> ATQRKGTDEIYGLGSLPSAGPGRWEYLANPGNWHPERRKLHEKLLDQARSSALTLAESLESDGCQPTLFALRGNTATGKTRIATKKIPVLAAALKKTAGKGCVNPDVFKSSLAKSETGAKIFSSAQVHSESSFLADRFEGGLRSQKTGSGAIASIVVDKRLSREYEIDSYIQLAKETGRKVELCDIDAPLENSLVGVLQRKPEGEDPRPPYPVVSSGFVAVRSNRMYVIDRFIADPSLGNYRLFGTAEDGEK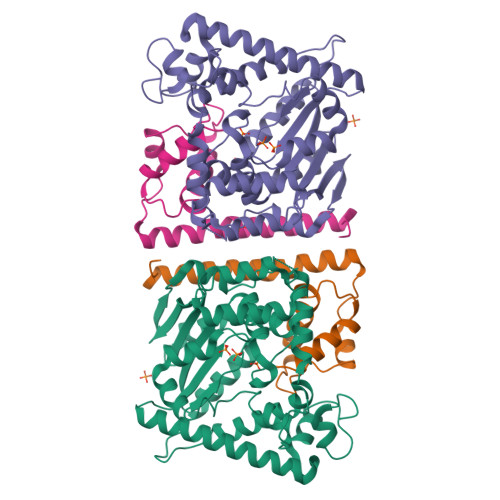VMVASVIGGEFSVENAELYEKITSPQLSVTGDLADKVIDKELIDRLENNIADPERAAKTRAALEKYSGKSWSAALAAHSELI;> MKTLTGADALEFHKKLKERNKALHASDLELALVHADAVGKERFDLEELEKICDTSDAGRLTDAKERNDIYERMYYVEYPNVMTLKEFAHIVETLFSWS> EKQVTKVKDTNIFPYTGVVAFKSATGFVVGKNTILTNKHVSKNYKVGDRITAHPNSDKGNGGIYSIKKIINYPGKEDVSVIQVEERAIERGPKGFNFNDNVTPFKYAAGAKAGERIKVIG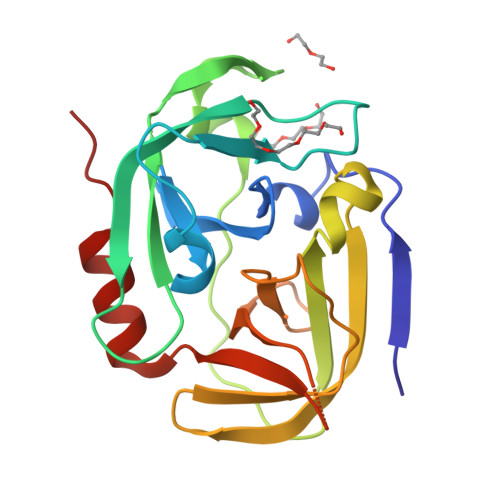YPHPYKNKYVLYESTGPVMSVEGSSIVYSAHTERGNSGSPVLNSNNELVGIHFASDVKNDDNRNAYGVYFTPEIKKFIAENIDKGS The ReAV enzyme from Rhizobium etli, a representative of Class 3 L-asparaginases, is sequentially and structurally different from other known L-asparaginases. Asparaginases (EC 3.5.1.1) catalyze the hydrolysis of L-asparagine, generating L-aspartate and ammonia. ReAV is a homodimeric protein, with each subunit containing a highly specific zinc-binding site created by two cysteines, a lysine, and a water molecule. Two Ser-Lys tandems (Ser48-Lys51, Ser80-Lys263) are located in the close proximity of the metal binding site, with Ser48 hypothesized to be the catalytic nucleophile.

The positively charged Arg47 side chain participates in salt-bridge interactions with the carboxylate side chains of Asp187, Asp267, and Glu17 from the adjacent protein chain, creating a network of H-bonds that supports the dimer structure. Furthermore, the crystal structure of the ReAV protein in complex with L-Asn showed that the guanidinium group of Arg47 stabilizes the position of the substrate α-carboxylate group. Thus, replacing the protonated Arg47 side chain with alanine disrupted the hydrogen bond network in this region, rendering the mutant protein inactive. The crystal structure of this mutant revealed that the absence of Arg47 caused only minor structural rearrangements and atomic shifts in the active site region, which were nearly identical in the four protein chains. The substitution of Arg47 by alanine affects the conformation of Glu17, which can no longer form H-bonds to the Nη atom of Arg47 of the complementary subunit. The metal binding site is conserved in the mutant structure and fully occupied with Zn2+. High difference electron density peaks were detected in the close vicinity of the Ser48 hydroxyl, as previously observed in both the ReAIV and ReAV crystal structures, and these peaks were interpreted as three water molecules forming very short H-bonds with the Ser48 Oγ atom (O…O 2.30–2.50 Å), as well as within their triangle (2.40–2.50 Å). The hydrogen bond network at the Ser-Lys tandems (Ser48-Lys51 and Ser80-Lys263) closely resembles that of the WT protein. Only one conformer of Asp187 is observed in the electron density maps, with one of its Oδ atoms forming an H-bond to the water molecule from the metal coordination sphere. The R47A mutant was inactive as well, due to its inability to anchor the L-Asn substrate in the active site.

>[4x]GIDPFTMTPSEDFVVTDRGGIVENSHRVHAAVVDAKGRLLYALGNPTRMTLAASAAKPAQALAILETEGVAGYGFDDADIALMCASHSSEDRHIARTRAMLSKIKAEEADLRCGGHPSLSEMVNRSWIKQDFIPTAVCSNCSGKHVGMLAGARAIGAGTDGYHLPDHPMQGRVKRTVAELCDLDAGDVEWGTDGCNLPTPAFPLDRLGRIYAKLASAADGSDAGEGQSTRCAALAHIFRAMARHPEMVAGEGRYCTMLMRAFDGALVGKLGADASYAIGVRASDATRQLGTDGALGISVKIEDGNLEMLYAVVTELLERLGIGSPDVRSQLASFHHPQRVNTMGVTTGGVSFPFKLRGSKSNVDDPRLAAVAR> XEAQ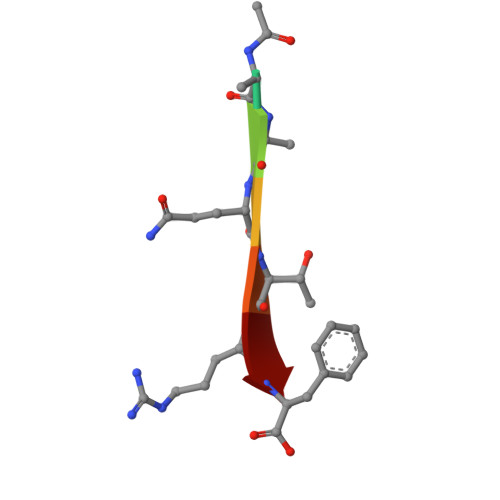TRF>MTSASNPPAFRLETSDGDEEGSAEVNKGKNEPPPMESPFQGEDRNFSPQIKVNLNYRKGLGPSQQDPNRFDRDRLFSVVSRGVPEELTGLLEYLRRTSKYLTDSAYTEGSTGKTCLMKAVLNLQDGVNACILPLLQIDRDSGNPQPLVNAQCTDEFYRGHSALHIAIEKRSLWCVKLLVENGANVHIRACGRFFQKHQGTCFYFGELPLSLAACTKQWDVVTYLLENPHQPASLEATDSLGNTVLHALVMIADNSPENSALVIHMYDSLLQMGARLCPTVQLEDICNHQGLTPLKLAAKEGKIEIFRHILQREFSGLYQPLSRKFTEWCYGPVRVSLYDLSSVDSWEKNSVLEIIAFHCKSPHRHRMVVLEPLNKLLQEKWDRLIPRFFFNFACYLVYMIIFTIVAYHQPSLEQPAIPSSKATFGDSMLLLGHILILLGGIYLLLGQLWYFWRRRLFIWISFMDSYFEILFLVQALLTVLSQVLRFVETEWYLPLLVSSLVLGWLNLLYYTRGFQHTGIYSVMIQKVILRDLLRFLLVYLVFLFGFAVALVSLSREARSPKAPEDSNTTVTEKPTLGQEEEPVPYGGILDASLELFKFTIGMGELAFQEQLRFRGVVLLLLLAYVLLTYVLLLNML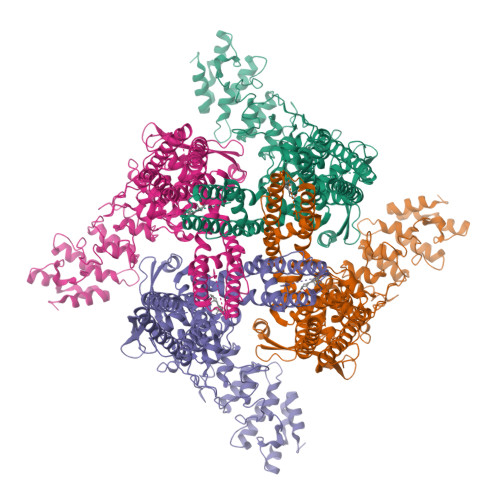IALMSETVNSVATDSWSIWKLQKAISVLEMENGYWWCRRKRHRAGRLLKVGTKGDGIPDERWCFRVEEVNWAAWEKTLPTLSEDPSGAGITGYKKNPTSKPGKNSASEEDHLPLQVLQSH[4x]>MALEPLKVEKFATANRGNGLRAVTPLRPGELLFRSDPLAYTVCKGSRGVVCDRCLLGKEKLMRCSQCRVAKYCSAKCQKKAWPDHKRECKCLKSCKPRYPPDSVRLLGRVVFKLMDGAPSESEKLYSFYDLESNINKLTEDKKEGLRQLVMTFQHFMREEIQDASQLPPAFDLFEAFAKVICNSFTICNAEMQEVGVGLYPSISLLNHSCDPNCSIVFNGPHLLLRAVRDIEVGEELTICYLDMLMTSEERRKQLRDQYCFECDCFRCQTQDKDADMLTGDEQVWKEVQESLKKIEELKAHWKWEQVLAMCQAIISSNSERLPDINIYQLKVLDCAMDACINLGLLEEALFYGTRTMEPYRIFFPGSHPVRGVQVMKVGKLQLHQGMFPQAMKNLRLAFDIMRVTHGREHSLIEDLILLLEECDANIRASEGHHHHHH[2x]

SET domain histone methyltransferases (HMTases) mediate epigenetic post-translational histone modifications that govern transcriptional activity, in part by modulating chromatin structure and accessibility of transcription factors and RNA polymerase II (pol Il) to promoters. SMYD3 and its 4 vertebrate paralogs derive from an ancient family of SET HMTases with orthologs present in plants, animals, fungi, and some (typically parasitic) protozoa. All SMYDs have the N-terminal terminal portion of SET (N-SET), followed by a Myeloid translocation protein 8, Nervy, and DEAF-1 (MYND) domain, N-terminal to an intermediate or linker sequence (I-SET) of variable length and configuration. We demonstrate that SMYD3 can function as a transcriptional repressor via MYND interactions as well as through hitherto undetected H4K20 HMTase activity.

We present here, in addition to the independent high resolution co-crystal structure of the full length human SMYD3 with the S-adenosyl methionine (SAM) analog Sinefungin, a detailed mutational and biochemical assessment of SMYD3 function. Baculoviral SMYD3 was co-crystallized with the SAM analog Sinefungin, and the structure was solved to 1.8 Å resolution. SMYD3-Sinefungin crystallized as 2 symmetry-related molecules/unit cell (P21). The domains comprising the “core” of the split-SET (N-SET, C-SET, post-SET) of SMYD3 and the MYND domains overlay with those of corresponding conventional domains. About one third of the SMYD3 substrate binding site is formed by the Intermediate SET spacer (I-SET) region located C-terminal to MYND. The peptide is bound in the conventional manner; i.e., the methyl-lysine is oriented on the opposite surface of SMYD3 from the SAM/Sinefungin methyl donor, with a narrow channel connecting the two surfaces of the SET domain. For example, residue F259 interacts with the adenine ring of Sinefungin and the Y239 of the aromatic cage, which itself packs against Y257. The SMYD3 CTD is a superhelical 9 α-helical bundle which constricts the floor of the substrate binding site opposite to the I-SET domain, preventing the trivial insertion of substrates. In fact, the CTD clamps further down on the peptide binding space of SMYD3 than of SMYD1, featuring a greater superhelical pitch, such that it contacts the MYND domain (circled region of Fig. 8). Close inspection of the overlay indicates that the H4 peptide forms part of the support for the SAM binding pocket in the SET8 structure, whereas the SAM binding pocket is fully formed and stabilized in SMYD3, independent of any substrate.CARBA-NICOTINAMIDE-ADENINE-DINUCLEOTIDE | C22 H30 N7 O13 P2 | 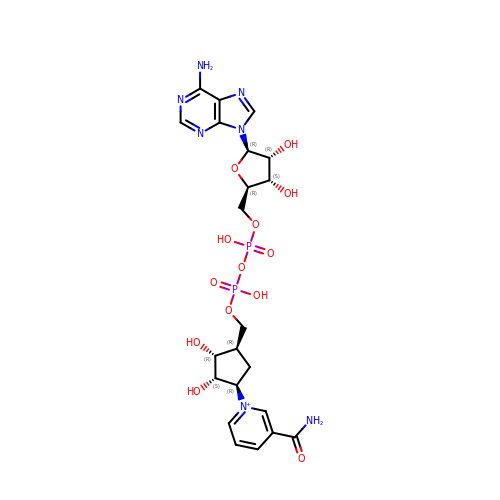DGPLSUKWXXSBCU-VGXGLJSLSA-O> SNAGTLQEYQKRMKKLDQQYRERIRNAELFLQLETEQVE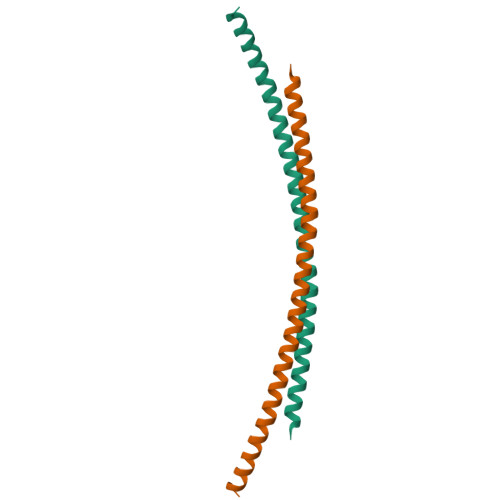RNYIKEKKAAVKEFEDKKVELKENLIAELEEKKKMIENEKLTMELTG>[8x]MALNVGPGGGSPVSTVEDTGRVELTPQEAAKVATTRCICYSTTQYVKDFLAGPMQKVFTDTYFVEPPLDKDTAQLARGYDVAVLFVNDRADASVIKELAKAGVKLIALRCAGFDRVDLHACAEHGVRVVRVPTYSPESVAEHAVALIFALNRHLTDAYIRVRMGNYSLSGLVGVEMRHKVVGVVGTGAIGQQAARILKGIGCKVFAYDIKPNPAVEAMGIPYVSLDELLAMSDIVTLHCPLLPSTRQLINKESIQKMKKGVMLINVSRGGLIDSAALFDALESGQIGALGLDVYENEGGLFFVDHTKFDPSVRMQKWDRQFRTLLSYPQVLVTPHTAFLTEEALNNICTTTIQNIADYVLDRPLGNEVKAQPAPAGKTLEHHHHHH

Of these, the most likely d-nLDH is Cre07.g324550, which shows 30–33% protein sequence identity to known d-nLDH sequences and possesses the NAD+-binding domain (GXGX2GX17D), and the conserved histidine (for catalysis), arginine (for substrate binding) and glutamic acid residues (for modulating pH dependence) characteristic of such enzymes. As expected from sequence comparisons, enzyme assays confirmed that the protein was a d-LDH with a preference for the reduction of pyruvate to d-lactate and a specificity for NADH. Consequently, we annotate Cre07.g324550 as Cr-LDH1. Our immunochemical analysis clearly showed that Cr-LDH1 was located in the chloroplast, consistent with the presence of a predicted chloroplast transit peptide.

To examine the enzymatic function of Cre07.g324550, a C-terminal His-tagged derivative was expressed in Escherichia coli using a codon-optimized synthetic gene. As the gene product was predicted by ChloroP (Emanuelsson et al. 1999, Emanuelsson et al. 2000) to be targeted to the chloroplast, the putative transit peptide of 44 residues was removed and only residues 45–421 were expressed. The 40 kDa His-tagged derivative was expressed as a soluble protein that could be isolated by Ni2+ affinity chromatography. The mass of the native species was determined to be approximately 200 kDa by size-exclusion chromatography, indicating the formation of an oligomer. Blue native (BN) gels indicated that the Cr-LDH1 holoenzyme had an apparent mass of >200 kDa, suggesting the formation of a larger complex in vivo. His-tagged recombinant Cr-LDH1 was crystallized and its structure determined by X-ray crystallography. There were eight copies of the monomer in the asymmetric unit, corresponding to two tetramers, as predicted by PISA. NAD+ molecules added during crystallization were observed in the active site of each monomer close to the conserved His378, Arg311 and Glu340 residues noted previously. Interestingly, recombinant His-tagged Cr-LDH1 also showed glyoxylate reductase activity, albeit with a lower catalytic efficiency, indicating a more wide-ranging role in metabolism than just the reduction of pyruvate. No activity was detected using NADPH or NADP+ (data not shown).> QAEEWYFGKITRRESERLLLNPENPRGTFLVRESETTKGAYCLS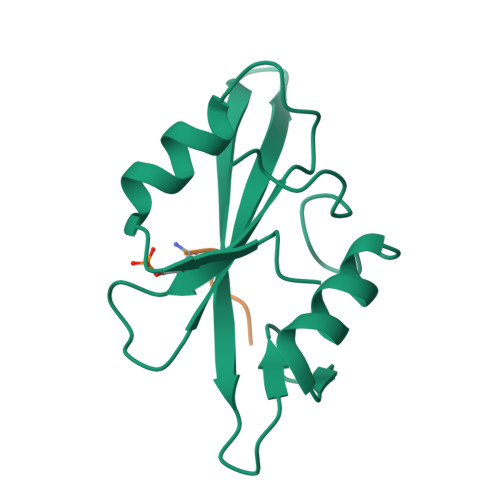VSDFDNAKGLNVKHYKIRKLDSGGFYITSRTQFSSLQQLVAYYSKHADGLCHRLTNVCPT;> YVPML> MSVLTKAIVNADAEARYLSPGELDRIKSFVASGERRLRIAQTLTEARERI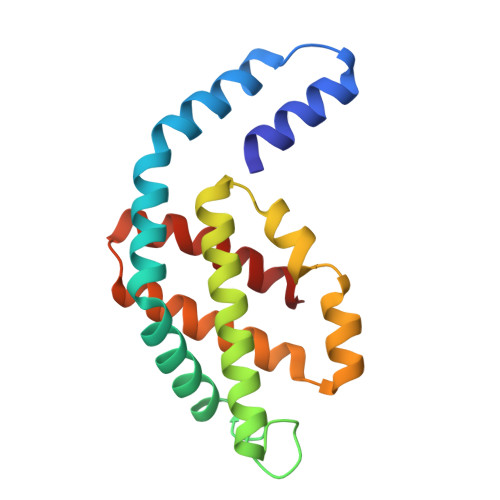VKQAGDQLFQIRPDVVSPGGNAYGEKMTALCLRDLDYYLRLVTYGIVAGDVTPIEEIGIIGVKEMYNSLQTPIPAVAEGVRAMKNVATSLLSGDDAAEAGFYFDYLVGAMQ>ASQNSFRIEYDTFGELKVPNDKYYGAQTVRSTMNFKIGGVTERMPTPVIKAFGILKRAAAEVNQDYGLDPKIANAIMKAADEVAEGKLNDHFPLVVWQTGSGTQTNMNVNEVISNRAIEMLGGELGSKIPVHPNDHVNKSQSSNDTFPTAMHIAAAIEVHEVLLPGLQKLHDALDAKSKEFAQIIKIGRTHTQDAVPLTLGQEFSGYVQQVKYAMTRIKAAMPRIYELAAGGTAVGTGLNTRIGFAEKVAAKVAALTGLPFVTAPNKFEALAAHDALVELSGAMNTTACSLMKIANDIRFLGSGPRSGLGELILPENEPGSSIMPGKVNPTQCEAMTMVAAQVMGNHVAVTVGGSNGHFELNVFKPMMIKNVLHSARLLGDASVSFTENCVVGIQANTERINKLMNESLMLVTA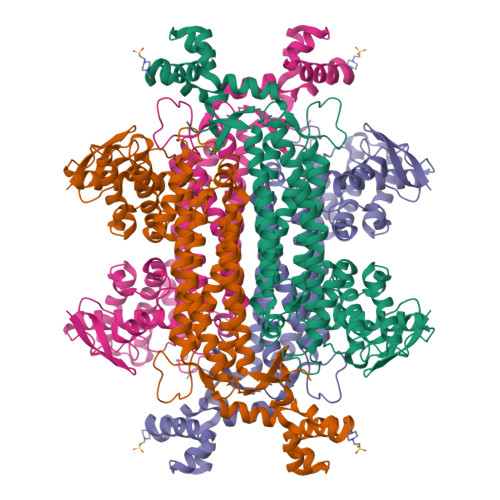LNPHIGYDKAAKIAKTAHKNGSTLKETAIELGYLTAEQFDEWVKPKDMLGPK[2x]>MSLINARLIAFEDQWVPALNAPLKQAILAD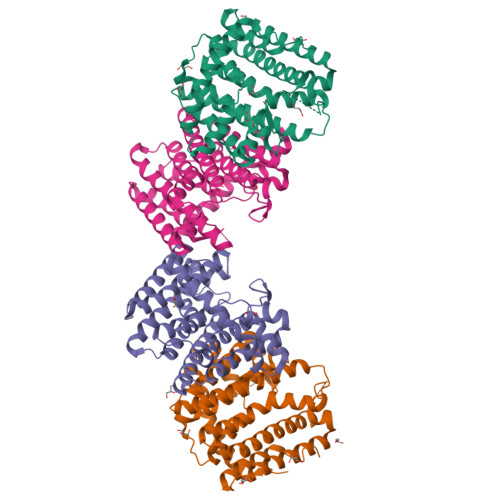SQDAQLAAAMTYSVLAGGKRLRPLLTVATMQSLGVTFVPERHWRPVMALELLHTYSLIHDDLPAMDNDALRRGEPTNHVKFGAGMATLAGDGLLTLAFQWLTATDLPATMQAALVQALATAAGPSGMVAGQAKDIQSEHVNLPLSQLRVLHKEKTGALLHYAVQAGLILGQAPEAQWPAYLQFADAFGLAFQIYDDILDVVSSPAEMGKATQKDADEAKNTYPGKLGLIGANQALIDTIHSGQAALQGLPTSTQRDDLAAFFSYFDTERVNEGHHHHHH[4x]> GSMEEEAETEEQQRFSYQQRLKAAVHYTVGCLCEEVALDKEMQFSKQTIAAISELTFRQCENFAKDLEMFARHAKRTTINTEDVKLLARRS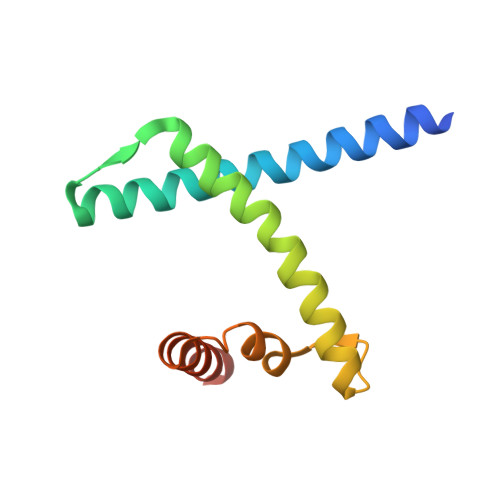NSLLKYITDKSEEIAQINLER> GSHMTDPRKNGDLHEPATAPATPWSKSELVRQLRDLGVRSGDMVMPHVSLRAVGPLADGPQTLVDALIEAVGPTGNILAFVSWRDSPYEQTLGH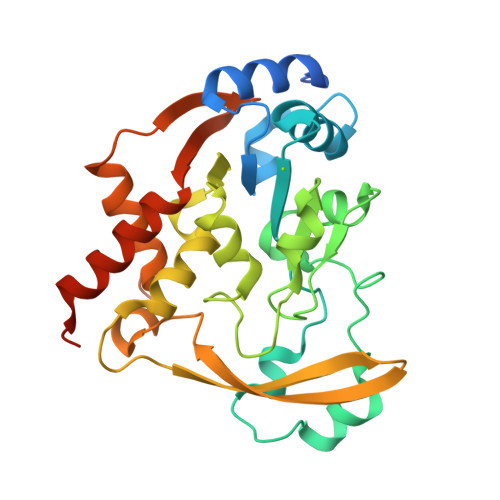DAPPAAIAQSWPAFDPDHAPAYPGFGAINEFIRTYPGCRRTAHPDASMAAIGPDAAWLVAPHEMGAAYGPRSPIARFLAHAGKILSIGAGPDAVTALHYAEAVARIEGKRRVTYSMPLLREGKRVWVTTSDWDSNGILDEYAAPDGPDAVERIARDYLARTRVAQGPVGGAQSRLIDAADIVSFGIEWLEARHAAPAAAALKPKQRRD>[3x]SGFVCNTCPEKWINFQRKCYYFGKGTKQWVHARYACDDMEGQLVSIHSPEEQDFLTKHASHTGSWIGLRNLDLKGEFIWVDGSHVDYSNWAPGAPTSRSQGEDCVMMRGSGRWNDAFCDRKLGAWVCDRLATCTPPASEGSAE

The second principal receptor for IgE, CD23, is a type II transmembrane glycoprotein with a C-type lectin-like domain (CTLD)4 (3, 4). In its membrane-bound form, CD23 consists of three CTLD “heads” connected to the membrane via a trimeric α-helical coiled-coil “stalk”. The interaction between CD23 and IgE is critical in the regulation of IgE synthesis, which can be up- or down-regulated depending on the oligomerization state of CD23 (2, 9, 10). We have determined the crystal structures of the human lectin-like head domain of CD23 in its Ca2+-free and Ca2+-bound forms, as well as the crystal structure of the Ca2+-bound head domain of CD23 in complex with a subfragment of IgE-Fc consisting of the dimer of Cϵ3 and Cϵ4 domains (Fcϵ3-4).

To verify that the principal site is indeed the location of Ca2+ binding to derCD23 in solution, and to confirm the exact nature of the interaction, several single point mutations in derCD23 were generated: conserved residues were mutated within the principal (E249A and D270A) and auxiliary (S252A and D258A) calcium-binding sites, along with the highly conserved Asn-269 residue (N269A and N269D). As expected, the two principal binding site derCD23 mutants, E249A and D270A, were unable to bind Ca2+. In contrast the E249A (principal site) mutant, which crystallized in yet another form, has cis Pro-250 in all three independent copies. Here also, loop 4 adopts a similar conformation to that observed in the Ca2+-bound derCD23 structure (and conformation 2 of the Ca2+-free and S252A structures). Mutation of the adjacent Glu-249, part of the EPT motif, to alanine appears to have locked Pro-250 into the cis configuration. Thus, of the 30 independent copies of derCD23 presented here, 19 are trans; of the remaining 11, four are cis as a result of the Ca2+ present, and 3 are cis as a result of mutation of the adjacent Glu-249.> GPSFPEPKVVRSQGGLLSLKLSATPTPLAIAGQRATLLTYGGSFPGPTLRVRPRDTVRLTLENRLPEPTNLHWHGLPISPKVDDPFLEIPPGESWTYEFTVPKELAGTFWYHPHLHGRVAPQLFAGLLGALVVESSLDAIPELREAEEHLLVLKDLALQGGRPAPHTPMDWMNGKEGDLVLVNGALRPTLVAQKATLRLRLLNASNARYYRLALQDHPLYLIAADGGFLEEPLEVSELLLAPGERAEVLVRLRKEGRFLLQALPYDRGAMGMMDMGGMAHAMPQGPSRPETLLYLIA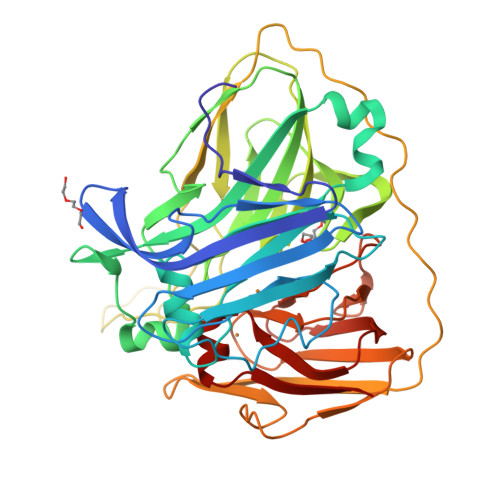PKNPKPLPLPKALSPFPTLPAPVVTRRLVLTEDMMAARFFINGQVFDHRRVDLKGQAQTVEVWEVENQGDMDHPFHLHVHPFQVLSVGGRPFPYRAWKDVVNLKAGEVARLLVPLREKGRTVFHCHIVEHEDRGMMGVLEVG> MGNQDKSKETSELDDLALPRSIIMRLVKGVLPEKSLVQKEALKAMINSATLF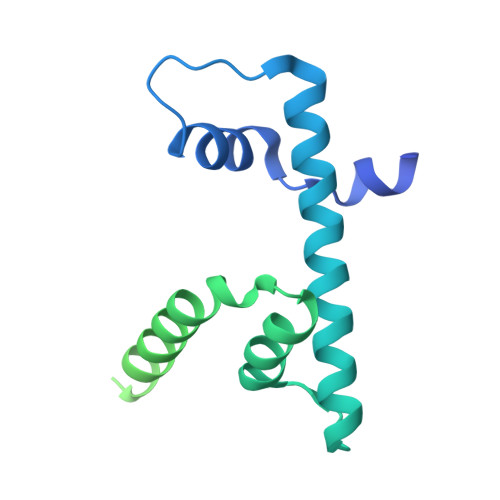VSFLTSASGEIATNNNRKILMPQDVLNALDEIEYPEFSKTLKKHLEAYELALKEKRLKLPNVSDVDNRKKAKIDAHDTTPLDEEKDELEEERIAEDIAQNEVEQNIDDVEDLEEVNDTLDANAESPQIETIHLTDATGNPIEDSSESDSEESLQLNDSSAAAENLYFQGLEDYKDDDDKHHHHHHHHHH> MKHHHHHHMKQNSPLDEENLTQENQDRGTHVDRGLASANVDFAFSLYKQLVLKAPDKNVIFSPLSISTALAFLSLGAHNTTLTEILKGLKFNLTETSEAEIHQSFQHLLRTLNQSSDELQLSMGNAMFVKEQLSLLDRFTEDAKRLYGSEAFATDFQDSAAAKKLINDYVKNGTRGKITDLIKDLDSQTMMVLVNYIFFKAKFEMPFDPQDTHQSRFYLSKKKYVMVPMMSLHHLTIPYFRDEELSCTVVQLNYTGNASALFILPDQDKMEEVEAMLSQETLSRFFESLEFREIGELYLPKFSISRDYNLNDILLQLGIE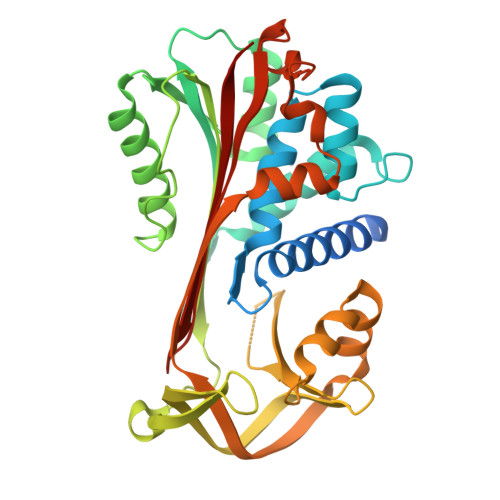EAFTSKADLSGITGARNLAVSQVVHKAVLDVFEEGTERSAATALEVLFQ>[11x]MAQVINTNTMSLNAQRNLSTSGSSLATTIQRLSSGSRINSAKDDAAGLAISERFGTQIRGTDVAIRNANDGISLAQVAEGSLTEIGNNLQRVRELSVQASNATNSASDRKALQAEVTQLVSEIDRVAKQSDFNGTKLLDGTFSSQLFQVGANAGQAIAIDKTIDAKAGSLGTSTFATGA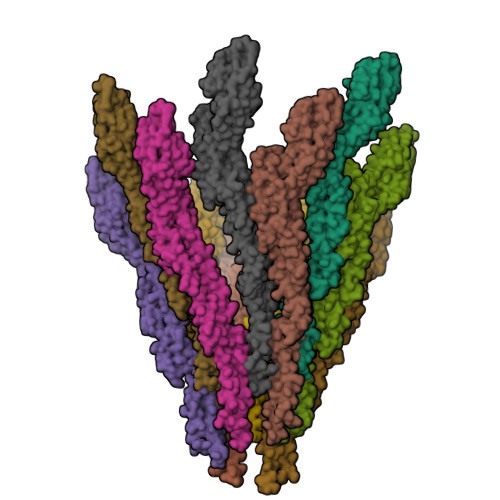TAALAASTDGARFSGTVMGVDIGTVEVKAGATTADASKAVATAINAKIGEAGIYAEANSDGTLKLSSVKEGKAVATADIALMRSDYDATAKTWGTAAAAGAYTAGTNTSANVQKLDVSTVLGAQQALEVVDKALGAINSTRADLGAIQNRFTSVVANLQTSSENLSASRSRIKDTDFAKETAELTRTQILQQAGTAMLAQANQVPQGVLSLLR> RDAQRMNILAGRIIAETVRSTLGPKGMDKMLVDDLGDVVVTNDGVTILREMSVEHPAAKMLIEVAKTQEKEVGDGTTTAVVVAGELLRKAEELLDQNVHPTIVVKGYQAAAQKAQELLKTIACEVGAQDKEILTKIAMTSITGKGAEKAKEKLAEIIVEAVSAVVDDEGKVDKDLIKIEKKSGASIDDTELIKGVLVDKERVS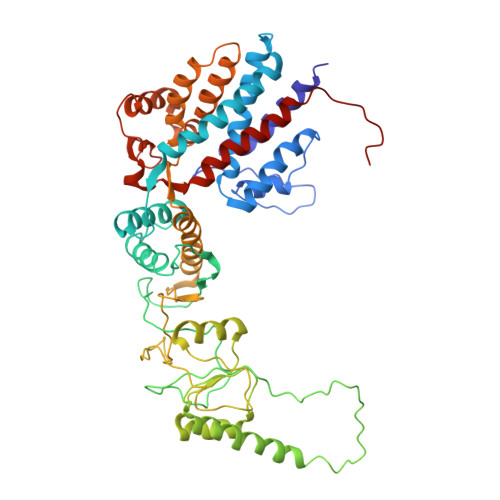AQMPKKVTDAKIALLNCAIEIKETETDAEIRITDPAKLMEFIEQEEKMLKDMVAEIKASGANVLFCQKGIDDLAQHYLAKEGIVAARRVKKSDMEKLAKATGANVITNIKDLSAQDLGDAGLVEERKISGDSMIFVEECKHPKAVTMLIRGTTEHVIEEVARAVDDAVGVVGCTIEDGRIVSGGGSTEVELSMKLREYAEGISGREQLAVRAFADALEVIPRTLAENAGLDAIEILVKVRAAHASNGNKCAGLNVFTGAVEDMCENGVVEPLRVKTQAIQSAAESTEMLLRIDDVIAAEKLR> ANNLGSKLLVGYWHNFDNGTGIIKLKDVSPKWDVINVSFGETGGDRSTVEFSPVYGTDADFKSDISYLKSKGKKVVLSIGGQNGVVLLPDNAAKDRFINSIQSLIDKYGFDGIDIDLQSGIYLNGNDTNFKNPTTPQIVNLISAIRTISDHYGPDFLLSMAPETAYVQGGYSAYGSIWGAYLPIIYGVKDKLTYIHVQHYNAGSGIGMDGNNYNQGTAD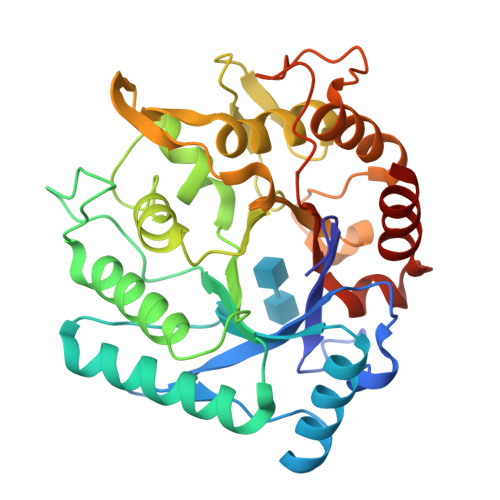YEVAMADMLLHGFPVGGNANNIFPALRSDQVMIGLPAAPAAAPSGGYISPTEMKKALNYIIKGVPFGGKYKLSNQSGYPAFRGLMSWSINWDAKNNFEFSNNYRTYFDGLSLQK>GPNPEGTLEAIKHTTSKISYYVNGKDHSTPAGQFMNQGTAAPDSIIHNGTTYVPVRMVSDLVGQPVYWEQASRTISLGLPVVKLYNAAGESVGSATLEQINDGVKVKITASGLTPGKHGFHVHENVIQGGDFKSAGGHFNPTDKHHGLENPQGSHVGDMPNLVVGTDGNAEAEMIIQHGTLEKDQPNTVLGRSLIIHAGEDDGVTDPSGNSGDRVAGGNIPE[2x]

pmcMost aerobes ranging from prokaryotes to eukaryotes are equipped with Cu/Zn-superoxide dismutase (CuZnSOD), which facilitates the disproportionation of superoxide into hydrogen peroxide and molecular oxygen. In order to become an active enzyme, CuZnSOD primarily needs to bind a copper ion at the copper-binding site because it functions as the active center for the disproportionation of superoxide. A structural significance of the S–S bond in CuZnSOD is to tether a loop to the protein core and thereby shape an entry site of the substrate O2− leading to the catalytic copper ion. Here, we found that a CuZnSOD protein in Paenibacillus lautus (PaSOD) has no Cys residue but exhibits a significant level of enzyme activity.

In contrast, we successfully solved the crystal structures of PaSOD-1 by the single-wavelength anomalous diffraction method using wavelengths of Cu and Zn absorption edges at 1.50 Å and 1.45 Å resolution, respectively. We used the structure from data collected at a wavelength of Zn absorption edge (1.275 Å) to discuss the PaSOD-1 structure unless otherwise noted. Furthermore, PaSOD was found to form a homodimer through the N-terminal domain with a novel protein fold. Furthermore, the α-helices from each of the subunits are held together by a hydrophobic cluster made of valine residues (V100, V102, V105, and V109) and thereby form an intersubunit two-helix bundle (right). PaSOD-1CTD assumes an immunoglobulin-like fold commonly observed for CuZnSOD, which is mainly composed of eight β-strands. PaSOD-1CTD was found to bind a copper and zinc ion, the positions of which were determined based upon the anomalous scattering data collected at wavelengths 1.373 Å (Cu signal) and 1.275 Å (Cu and Zn signals). Their binding sites are almost overlapped with those in hSOD1 and EcSodC; a copper ion in PaSOD-1CTD is ligated through His168, His170, His185, and His244, whereas a zinc ion through His185, His193, His202, and Asp205. His185 is a so-called bridging ligand binding both a copper and zinc ion. Reduction of the S–S bond is known to significantly decrease the conformational stability of both hSOD1 (21) and EcSodC; therefore, we wondered how PaSOD-1 lacking the S–S bond maintains the interaction between loop IV and the β8 strand. When we looked on loop IV–β8 strand interaction from the direction pointed by a red arrow in Figure 6, A and B, the S–S bond in hSOD1 was found to be replaced with a phenyl group of Phe179 and a hydrogen of Gly264 in PaSOD-1. Moreover, Asp52 in loop IV of hSOD1 points outward but is replaced with Ile174 pointing inward in PaSOD-1, where a hydrophobic cluster (Ile174, Gly176, Gly177, Phe179, Gly264, and Gly265) is formed between loop IV and β8 strand. Another notable feature in PaSOD-1 is that the side chain carbonyl and amide groups of Asn266 form hydrogen bonds with the main chain amide and carbonyl group of Ile174, respectively, whereas these hydrogen bonding interactions are missing in hSOD1.N-(2-fluorophenyl)-1H-pyrazolo[3,4-d]pyrimidin-4-amine | C11 H8 F N5 | 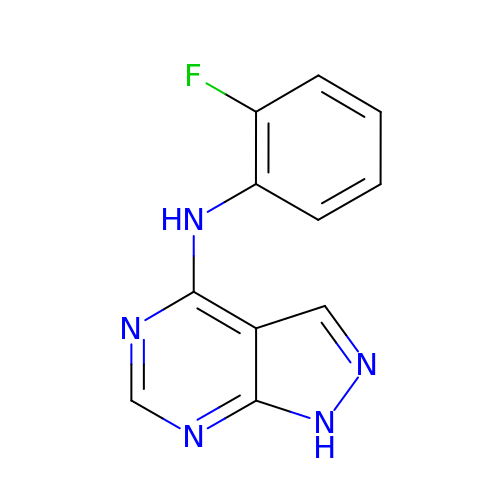MEYYGZBRFGDWPZ-UHFFFAOYSA-N>[3x]MAPSAYALDRSSVPSGKPRLMEGAESKARAGARKIHHLKIHGFDRVFGPGTHRWQRALWFAGVVFCFGISAHQIAMHVLDYLSEPVAVRIDFVAQNELRIPEITVCPRIFQQNTIFT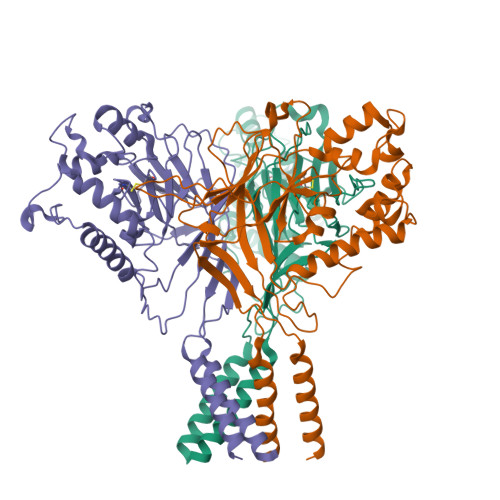DMVEKQGIDKMKFLDLIDRPEYDIMAVWNLSRIFSDNVSCSAHEGSSIISGSYVDPNMSQPHLVYTTSGQCINIPASRPLIYRGVNTFVRITDSQPRNLDEVRPEAIQIYFHEHHHAHLSRYLTGLRGYIVPIANPFAFSIRFTQINYANKTDSPCVDSEEYAACVEDFIEQRIYEKAQVQCRLPYMRPKLPLCSTPTDARKIFVATDDVIQNFEKESSCKRKCEETLYIVEFMHLFERSNISIDMSVYFAYNYIQVATEYLTYTLRGLLSDIGGVLGLFLGICILSVIEVFEVVIFSLQRVLCNEDKKQQNNE>[2x]AMARVGVLGAKGKVGATMVRAVA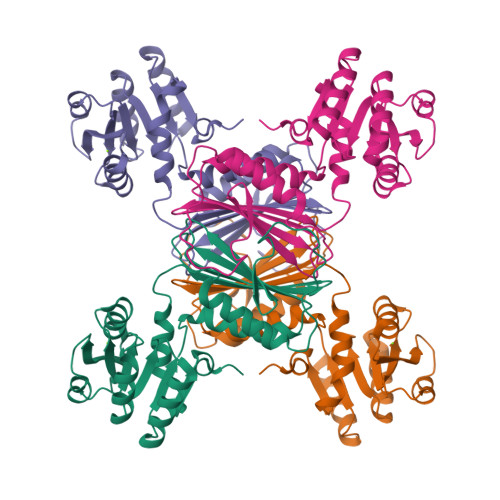AADDLTLSAELDAGDPLSLLTDGNTEVVIDFTHPDVVMGNLEFLIDNGIHAVVGTTGFTAERFQQVESWLVAKPNTSVLIAPNFAIGAVLSMHFAKQAARFFDSAEVIELHHPHKADAPSGTAARTAKLIAEARKGLPPNPDATSTSLPGARGADVDGIPVHAVRLAGLVAHQEVLFGTEGETLTIRHDSLDRTSFVPGVLLAVRRIAERPGLTVGLEPLLDLH>MAAVSGKSEAAEIEAGDRLDALRDQLQRYETPIIQTILARSALGGRAPSEQDEVRAALSRNAFEPSEVISEWLQTESGARFRSTRPLPPAVEFITPVVLSRDTVLDKPVVGKGIFPIGRRPQDPTNMDEFLDTSLLSLNQSSTVDLASAVSLDVSLLHLVSARVLLGYPIALAKFDWLHDNFCHILTNTTLSKSQKLANIIQQLTDHKQEVNVLSRVEQKSKSLSHLFRNDIPYPPHTQDRILRLFQAYLIPITTQIEAAAILDHANKC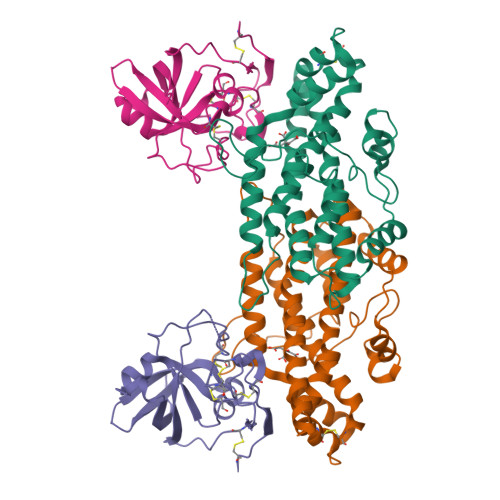TLEHHHHHH[4x];>MFPYRSLLQTCQPSGSIQGRSGNCNTENGSECCKNGRRYTTYGCSPPVTGSTRAVLTLNSFAEGGDGGGAAACTGKFYDDSKKVVALSTGWYNGGSRCRKHIMIHAGNGNSVSALVVDECDSTVGCDKDHNFEPPCRNNIVDGSPAVWDALGLNKDDGQAQITWSDELEHHHHHH[4x]> GTTSQKHRDFVAEPMGEKPVGSLAGIGEVLGKKLEERGFDKAYVVLGQFLVLKKDEDLFREWLKDTAGANAK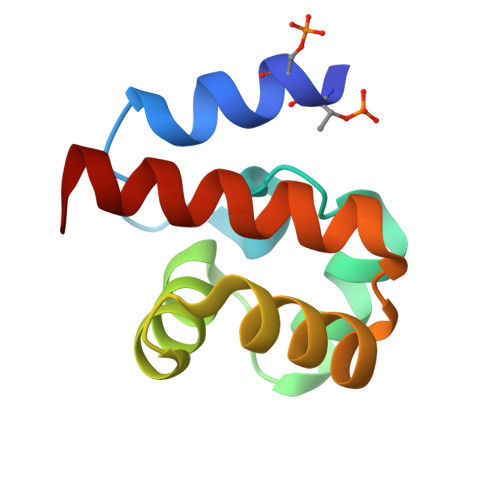QSRDAFGALREWADAFL>GHMEHRGTDIISLSQAATKIHQAQQTLQSTPPISEENNDERTLARQQLTSSLNALAKSGVSLSAEQNENLRSAFSAPTSALFSASPMAQPRTTISDAEIWDMVSQNISAIGDSYLGVYENVVAVYTDFYQAFSDILSKMGGWLLPGKDGNTVKLDVTSLKNDLNSLVNKYNQINSNTVLFPAQSGSGVKVATEAEARQWLSELNLPNSSLKSYGSGYVVTVDLTPLQK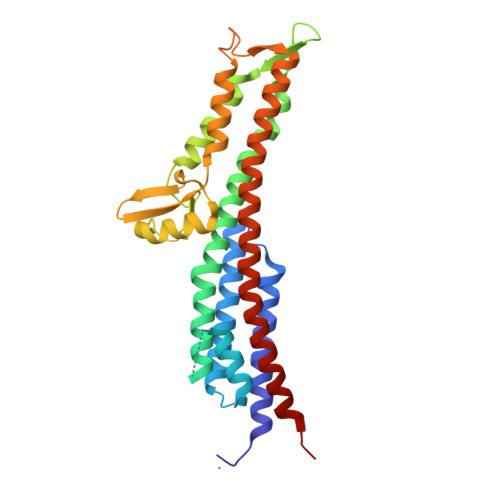MVQDIDGLGAPGKDSKLEMDNAKYQAWQSGFKAQEENMKTTLQTLTQKYSNANSLYDNLVKVLSSTISSSLETAKSFLQG[2x]>ALVFFAEDCGSNKCAII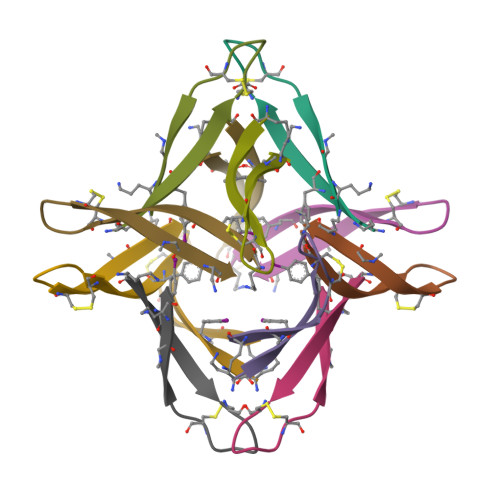GLAV[6x]N-{3-[4-(3-AMINO-PROPYL)-PIPERAZIN-1-YL]-PROPYL}-3-NITRO-5-(GALACTOPYRANOSYL)-BETA-BENZAMIDE | C23 H37 N5 O9 | 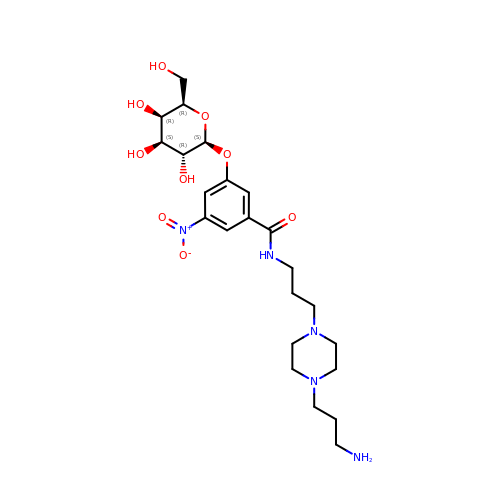UEIGEWJJVQHIAX-DLBZZEGUSA-N>MASAQAVGQGERGHFVLKSGHTIPAVGLGTWRAGSDTAHSVRTAIAEAGYRHVDTAAQYGVEKEVGRGLKAAMEGGINRKDLFVTSKLWCTELAPDRVRPALEKTLKDLQLDYLDLYLIHWPFRLKDGAHMPPEAGEVLELDMEGVWREMEGLVKDGLVKDIGVCNYTVAKLNRLMRSANVPPAVCQMEMHPGWKNDRIFEACKKHGIHVTAYSPLGSSEKNLAHDPLVEKVANKLDKTPGQVLLRWALQRGTSVIPKSTRDERIKENIQVFGWEIPEEDFRALCGIKDEKRVLTGEELFVNKTHGPYKSATEVWDHEDLEHHHHHH[2x]

Aldo-keto reductases (AKRs) are ubiquitous in nature and are able to reduce a wide range of substrates, from simple sugars to potentially toxic aldehydes. The AKR superfamily consists of generally monomeric proteins, typically ranging from 30 to 40 kDa, that are NAD(P) (H)-dependent and share a common (α/β)8-or TIM-barrel (triose phosphate isomerase). Recombinant ZmAKR4C13 efficiently reduced methylglyoxal and small aldehydes but showed poor activity toward aldoses larger than four carbons. The maize ZmAKR4C13 can thus detoxify small-aldehyde stress metabolites and is expressed at sites and times in embryos conducive to a role in stress tolerance and possible signaling.

To identify mechanistic features potentially affecting activity and roles of the ZmAKR4C13, we solved its crystal structure in two space groups at a resolution of 2.3 Å (P212121) and 1.45 Å (P21), respectively. The protein folds into a (α8/β8)-barrel with two additional α-helices (H1 and H2) packed against the α7-helix from the barrel. The residues Asp54, Tyr59, Lys87, and His120 correspond to the typical catalytic tetrad of AKRs according to structural comparison with the well characterized AKR1C9 (64). Although two and four monomers compose the asymmetric unit of the P21 and P212121 crystals, respectively, analysis of their interfaces using the PDBePISA program did not indicate formation of stable quaternary structures in solution. Two molecules of ethylene glycol were found at the substrate-binding site for ZmAKR4C13, allowing us to identify additional points of potential substrate anchoring based on hydrophobic interactions and hydrogen bonds. The first molecule occupies the same binding site as does acetate in the P212121 crystal and that of butanol in HvALR1. Replacement of a cysteine by the bulkier leucine at position 294∗ from Loop C seems to hamper the binding of C3-OH groups that are in the same orientation observed for glyceraldehyde in HsAKR1B1. Supporting this hypothesis, the orientation of the second ethylene glycol molecule bound in the ZmAKR4C13 active site displays an angular shift compared to the first one. Relative orientations of the two ethylene glycol molecules, which approximate aldose fragments, support the interpretation that Leu294∗ prevents longer C3-aldoses from adopting a conformation favorable for catalysis. Analysis of the active site, its modifications, and interaction with alternate substrates, indicates that the spatial bulk of Leu at position 294∗ of ZmAKR4C13 is instrumental to preventing aldoses with 4-C or more from serving as effective substrates under physiologically relevant conditions.>[2x]THFGVKYELWQPECELTAELRKTAGVAKMKV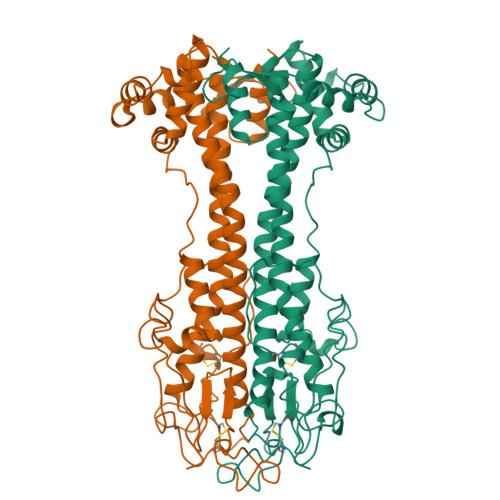NSDLNSFKTLELTKMKLLTFAAKFPESKEALTLRALEAALNTDLRALRDNIANGIDRAVRATAYASEAAGALFSGIQTLHDATDGTTYCLSASGQGSNGNAAMASQGCKPLALPELLTEDSYNTDVISDKGFPKISPLTNAQGQGKSGECGLFQAASGAQATNTGVQFSGGSRINLGLGAIVASAAQQPTRPDLSDFSGTARNQADTLYGKAHASITELLQLAQGPKPGQTEVETMKLLAQKTAALDSIKFQLAASTGKKTSDYKEDENLKTEYFGKTESNIEALWNKVKEEKVKGADPEDPSKESKISDLNTEEQLQRVLDYYAVA>GAMDPEFPSLEQDDEDEETRMVIVGKISFCPKDVLGHGAEGTIVYKGMFDNRDVAVKRILPECFSFADREVQLLRESDEHPNVIRYFCTEKDRQFQYIAIELCAATLQEYVEQKDFAHLGLEPITLLHQTTSGLAHLHSLNIVHRDLKPHNILLSMPNAHGRIKAMISDFGLCKKLAVGRHSFSRRSGVPGTEGWIAPEMLSEDCKDNPTYTVDIFSAGCVFYYVISEGYHPFGKSLQRQANILLGACNLDCFHSDKHEDVIARELIEKMIAMDPQQRPSAKHVLKHPFFWSLEKQLQFFQDVSDRIEKEALDGPIVRQLERGGRAVVKMDWRENITVPLQTDLRKFRTYKGGSVRDLLRAMRNKKHHYRELPVEVQETLGSIPDDFVRYFTSRFPHLLSHTYQAMELCRHERLFQTYYWHEPTEPQPPVI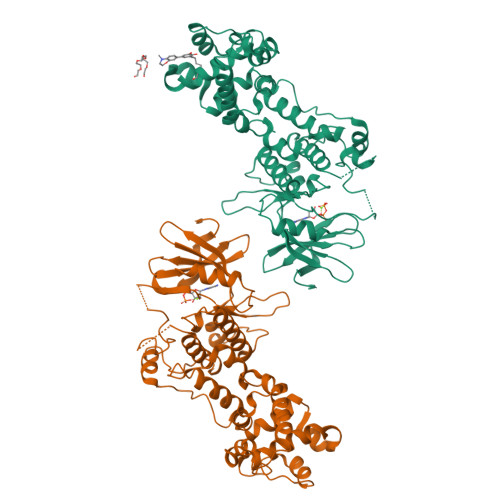PYAL[4x]> PPKELVNEWSLKIRKEMRVVDRQIRDIQREEEKVKRSVKDAAKKGQKDVCIVLAKEMIRSRKAVSKLYASKAHMNSVLMGMKNQLAVLRVAGSLQKSTEVMKAMQSLV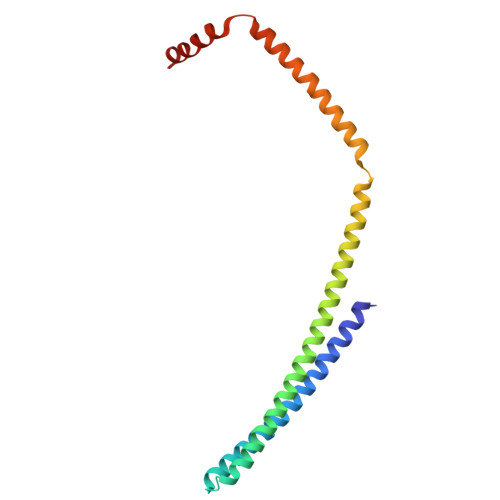KIPEIQATMRELSKEMMKAGIIEEMLEDTFESMDDQEEMEEEAEMEIDRIL> MDYKDDDDKGDHNHRHKHGDPLEVLFQGPGGDPHMSRESNDTIQSDTVRSSSKSDYFRIQLNNQDYYMSKPTFLDPSHGESLPLNQFSQVPNIRVFGALPTGHQVLCHVHGILPYMFIKYDGQITDTSTLRHQRCAQVHKTLEVKIRASFKRKKDDKHDLAGDKLGNLNFVADVSVVKGIPFYGYHVGWNLFYKISLLNPSCLSRISELIRDGKIFGKKFEIYESHIPYLLQWTADFNLFGCSWINVDRCYFRSPVLNSILDIDKLTINDDLQLLLDRFCDFKCNVLSRRDFPRVGNGLIEIDILPQFIKNREKLQHRDIHHDFLEKLGDISDIPVKPYVSSARDMINELTMQREELSLKEYKEPPETKRHVSGHQWQSSGEFEAFYKKAQHKTSTFDGQIPNFENFIDKNQKFSAINTPYEALPQLWPRLPQIEINNNSMQDKKNDDQVNASFTEYEICGVDNENEGVKGSNIKSRSYSWLPESIASPKDSTILLDHQTKYHNTINFSMDCAMTQNMASKRKLRSSVSANKTSLLSRKRKKVMAAGLRYGKRAFVYGEPPFGYQDILNKLEDEGFPKIDYKDPFFSNPVDLENKPYAYAGKRFEISSTHVSTRIPVQFGGETVSVYNKPTFDMFSSWKYALKPPTYDAVQKWYNKVPSMGNKKTESQISMHTPHSKFLYKFASDVSGKQKRKKSSVHDSLTHLTLEIHANTRSDKIPDPAIDEVSMIIWCLEEETFPLDLDIAYEGIMIVHKASEDSTFPTKIQHCINEIPVMFYESEFEMFEALTDLVLLLDPDILSGFEIHNFSWGYIIERCQKIHQFDIVRELARVKCQIKTKLSDTWGYAHSSGIMITGRHMINIWRALRSDVNLTQYTIESAAFNILHKRLPHFSFESLTNMWNAKKSTTELKTVLNYWLSRAQINIQLLRKQDYIARNIEQARLIGIDFHSVYYRGSQFKVESFLIRICKSESFILLSPGKKDVRKQKALECVPLVMEPESAFYKSPLIVLDFQSLYPSIMIGYNYCYSTMIGRVREINLTENNLGVSKFSLPRNILALLKNDVTIAPNGVVYAKTSVRKSTLSKMLTDILDVRVMIKKTMNEIGDDNTTLKRLLNNKQLALKLLANVTYGYTSASFSGRMPCSDLADSIVQTGRETLEKAIDIIEKDETWNAKVVYGDTDSLFVYLPGKTAIEAFSIGHAMAERVTQNNPKPIFLKFEKVYHPSILISKKRYVGFSYESPSQTLPIFDAKGIETVRRDGIPAQQKIIEKCIRLLFQTKDLSKIKKYLQNEFFKIQIGKVSAQDFCFAKEVKLGAYKSEKTAPAGAVVVKRRINEDHRAEPQYKERIPYLVVKGKQGQLLRERCVSPEEFLEGENLELDSEYYINKILIPPLDRLFNLIGINVGNWAQEIVKSKRASTTTTKVENITRVGTSATCCNCGEELTKICSLQLCDDCLEKRSTTTLSFLIKKLKRQKEYQTLKTVCRTCSYRYTSDAGIENDHIASKCNSYDCPVFYSRVKAERYLRDNQSVQREEALISLNDW;>[2x]MNRWVEKWLRVYLKCYINLILFYRNVYPPQSFDYTTYQSFNLPQFVPINRHPALIDYIEELILDVLSKLTHVYRFSICIINKKNDLCIEKYVLDFSELQHVDKDDQIITETEVFDEFRSSLNSLIMHLEKLPKVNDDTITFEAVINAIELELGHKLDRNRRVDSLEEKAEIERDSNWVKCQEDENLPDNNGFQPPKIKLTSLVGSDVGPLIIHQFSEKLISGDDKILNGVYSQYEEGESIFGSLF;> GPGGDLHMDALLTKFNEDRSLQDENLSQPRTRVRIVDDNLYNKSNPFQLCYKKRDYGSQYYHIYQYRLKTFRERVLKECDKRWDAGFTLNGQLVLKKDKVLDIQGNQPCWCVGSIYCEMKYKPNVLDEVINDTYGAPDLTKSYTDKEGGSDEIMLEDESGRVLLVGDFIRSTPFITGVVVGILGMEAEAGTFQVLDICYPTPLPQNPFPAPIATCPTRGKIALVSGLNLNNTSPDRLLRLEILREFLMGRINNKIDDISLIGRLLICGNSVDFDIKSVNKDELMISLTEFSKFLHNILPSISVDIMPGTNDPSDKSLPQQPFHKSLFDKSLESYFNGSNKEILNLVTNPYEFSYNGVDVLAVSGKNINDICKYVIPSNDNGESENKVEEGESNDFKDDIEHRLDLMECTMKWQNIAPTAPDTLWCYPYTDKDPFVLDKWPHVYIVANQPYFGTRVVEIGGKNIKIISVPEFSSTGMIILLDLETLEAETVKIDI;> MDQKASYFINEKLFTEVKPVLFTDLIHHLKIGPSMAKKLMFDYYKQTTNAKYNCVVICCYKDQTIKIIHDLSNIPQQDSIIDCFIYAFNPMDSFIPYYDIIDQKDCLTIKNSYELKVSESSKIIERTKTLEEKSKPLVRPTARSKTTPEETTGRKSKSKDMGLRSTALLAKMKKDRDDKETSRQNELRKRKEENLQKINKQNPEREAQMKELNNLFVEDDLDTEEVNGGSKPNSPKETDSNDKDKNNDDLEDLLETTAEDSLMDVPKIQQTKPSETEHSKEPKSEEEPSSFIDEDGYIVTKRPATSTPPRKPSPVVKRALSSSKKQETPSSNKRLKKQGTLESFFKRKAK

Assembled from catalytic Rev3 and accessory Rev7, Pol31, and Pol32 subunits, the translesion DNA synthesis (TLS) polymerase ζ (Polζ) plays an important role in the replication of damaged or mismatched DNA in eukaryotic cells, and in the prevention of cancer. The B-family multi-subunit DNA polymerase ζ (Polζ) is important for translesion DNA synthesis (TLS) during replication, due to its ability to extend synthesis past nucleotides opposite DNA lesions and mismatched base pairs. The structures decrypt a pentameric ring-like architecture for Polζ, with the catalytic Rev3 and the accessory Pol31, Pol32, and two Rev7 subunits (Rev7A and Rev7B) forming a daisy chain of protein-protein interactions. Rev3 makes contacts to the DNA via its palm, fingers, thumb, exonuclease, and N-terminal (NTD) domains.

We present here, at a nominal resolution of 3.05 Å, a cryo-EM structure of Polζ with an A:C mismatch at the primer terminus. The Rev3, Rev7A, Rev7B, Pol31, and Pol32 subunits are organized around the mismatched duplex DNA in the same pentameric ring-like architecture as the matched complex, with catalytic Rev3 alone making all of the contacts to the DNA. The structure shows how the Polζ active site responds to the mismatched duplex DNA distortion, including the loosening of key protein-DNA interactions and a fingers domain in an “open” conformation, while the incoming dCTP is still able to bind for the extension reaction. Amongst the various hydrogen bonding schemes that have been considered for an A:C mismatch within a DNA duplex, the DNA cryo-EM density we observe is most consistent with a “wobble” base pairing, in which the N6 and N1 atoms of adenine make putative hydrogen bonds with N3 and O2 atoms of cytosine, respectively. For the wobble pairing, the cytosine base shifts towards the major groove by ~1.2 Å, and the A:C base pair as a whole is much more propeller twisted (−17.8°) than the G:C base pair (−3.8°) in the matched complex. An open fingers domain creates space above the nascent G:C base pair and many of the van der Waals contacts observed in the matched complex are lost, including those from Leu1087 and Val1091 of the fingers helix αxB. The dCTP is anchored loosely in the active site by inter-base hydrogen bonds with templating G, and by the contact it maintains with the palm domain, including stacking interactions between its sugar and Tyr980, and hydrogen bonds between its β- and γ-phosphates and the main chain amides of Leu979 and Ser978, respectively. Of the two metals “A” and “B” observed in the active site of the matched complex7 and associated with a two-metal ion mechanism of catalysis, only metal B, a Ca2+ ion, appears to be coordinated to the dCTP triphosphate moiety.> MSMIDEPLYPIAVLIDELKNDDIQLRLNSIRRLSTIARALGEERTRKELIPFLSENNDDDDEVLLAMAEELGVFIPYVGGVEYAHVLLPPLETLSTVEETCVREKAVESLCRVGSQMRESDLVDHFISLVKRLAAGEWFTARVSACGVFHIAYPSAPDMLKTELRSLYTQLCQDDMPMVRRAAATNLGKFAATVESAHLKTDVMSMFEDLTQDDQDSVRLLAVEGCAALGKLLEPQDCVQHILPVIVNFSQDKSWRVRYMVANQLYELCEAVGPEPTRTEL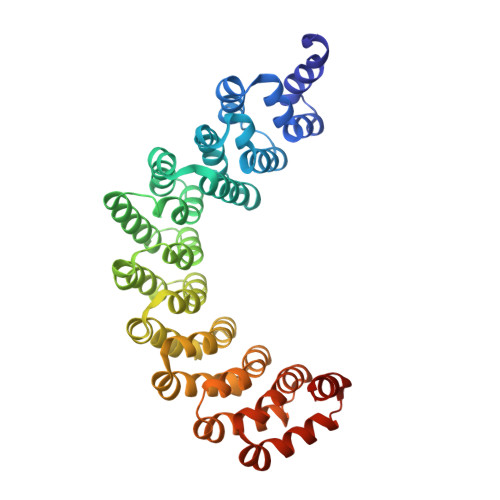VPAYVRLLRDNEAEVRIAAAGKVTKFCRILNPEIAIQHILPCVKELSSDSSQHVRSALASVIMGMAPVLGKDATIEHLLPIFLSLLKDEFPDVRLNIISKLDQVNQVIG> MLECTLVADAASGQELYRKGACDKAFAPMSTFKVPLAVMGYDAGILVDAH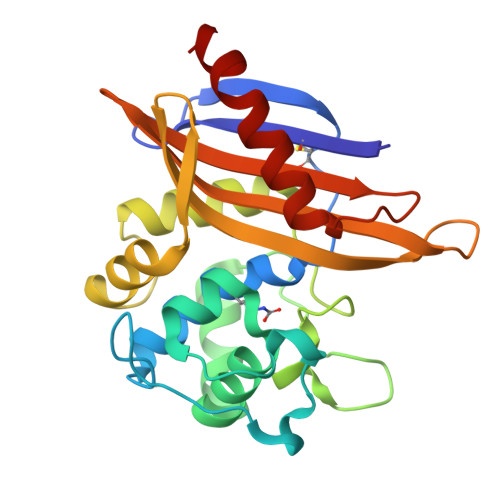NPRWDYKPEFNGYAFQQKTTDPTIWEKDSIVWYSQQLTRKMGQKRFAAYVAGFGYGNGDISGEPGKSNGLTHSWLGSSLKISPEGQVRFVRDLLSAKLPASKDAQQMTVSILPHFAAGDWAVQGKTGTGSFIDARGAKAPLGWFIGWATHEERRVVFARMTAGGAAGAQPAGPAARDAFLKALPDLAKAF> AKCVSYGVAQIKAPALHSQGYTGSNVKVAILGTGIDSSHPDLNVAGGASFVPSE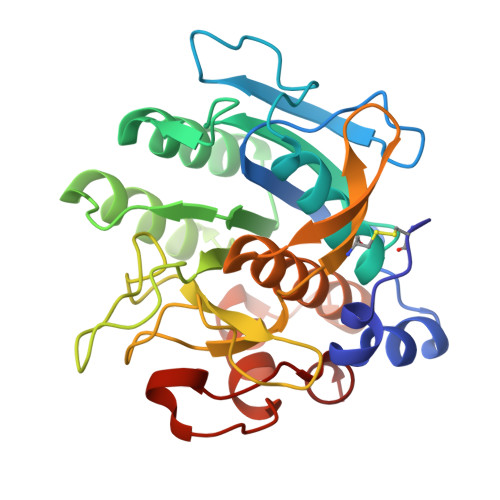TNPFQDNSSHGTHIAGTVLAVAPSASLYAVKVLGADGSGQASWVINGIEWAIANNMDVINMSLGSPSGSAALKAAVDKAVASGVVVVAAAGNSGTSGSSSTVTYPAKYPSVIAVGAVDSSNQRAPFSSVGPELDVMAPGVSICSTLPGGKYGALSGTSMASPHVAGAAALILSKHPNWTNTQVRSSLENTATKLGDSFYYGKGLINVEAAAQ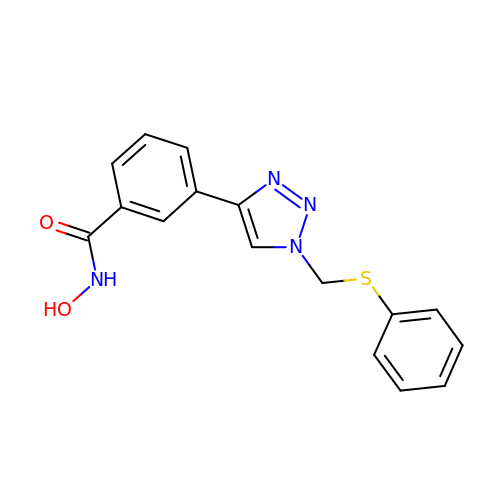~{N}-oxidanyl-3-[1-(phenylsulfanylmethyl)-1,2,3-triazol-4-yl]benzamide | C16 H14 N4 O2 S | DORPIZJGSLWDIY-UHFFFAOYSA-N~{N}-cyclopropyl-3-methyl-2~{H}-pyrazolo[4,3-d]pyrimidin-7-amine | C9 H11 N5 | 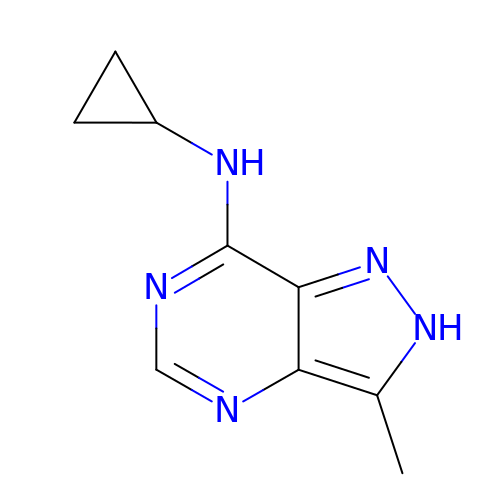CTRMXAARLMLINT-UHFFFAOYSA-N> GLNFPTYDGKDRVVSLSEKNFKQVLKKYDLLCLYYHEPVSSDKVTQKQFQLKEIVLELVAQVLEHKAIGFVMVDAKKEAKLAKKLGFDEEGSLYILKGDRTIEFDGEFAADVLVEFLLDLIEDPVEIISSKLEVQAFERIEDYIKLIGFFKSEDSEYYKAFEEAAEHFQPYIKFFATFDKGVAKKLSLKMNEVDFYEPFMDEPIAIPNKPYTEEELVEFVKEHQRPTLRRLRPEEMFETWEDDLNGIHIVAFAEKSDPDGYEFLEILKQVARDNTDNPDLSILWIDPDDFPLLVAYWEKTFKIDLFRPQIGVVNVTDADSVWMEIPDDDDLPTAEELEDWIEDVLSGKINTEDDDEDDD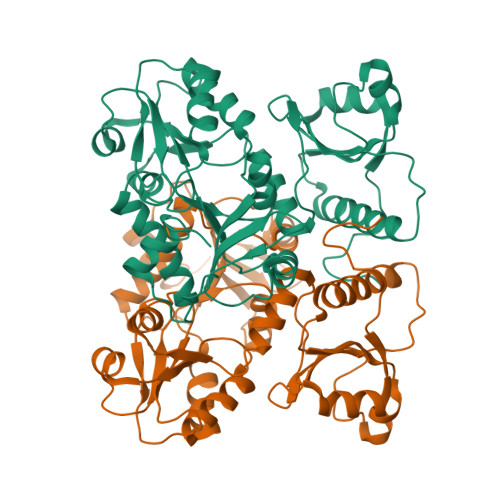DDDNSDEEDNDDSDDDDDE>HHHHHHHHGGLVPRGSHGGSMTDRLKGKVAIVTGGTLGIGLAIADKFVEEGAKVVITGRHADVGEKAAKSIGGTDVIRFVQHDASDEAGWTKLFDTTEEAFGPVTTVVNNAGIAVSKSVEDTTTE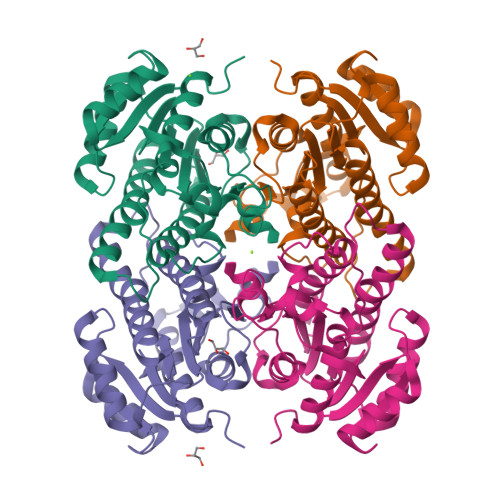EWRKLLSVNLDGVFFGTRLGIQRMKNKGLGASIINMSSISGFVGDPTLGAYNASKGAVRIMSKSAALDCALKDYDVRVNTVHPGYIKTPLVDDLEGAEEMMSQRTKTPMGHIGEPNDIAWICVYLASDESKFATGAEFVVDGGYTAQ[2x]> MASSRCPAPRGCRCLPGASLAWLGTVLLLLADWVLLRTALPRIFSLLVPTALPLLRVWAVGLSRWAVLWLGACGVLRA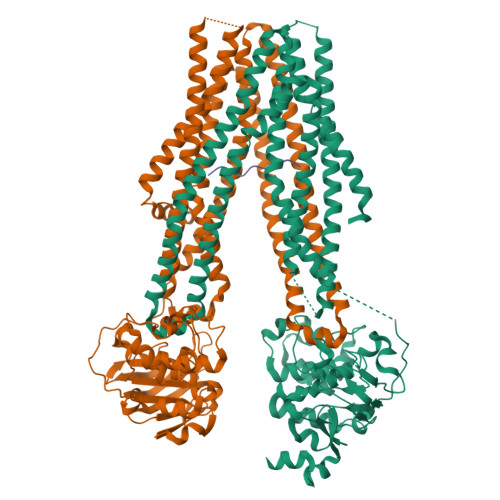TVGSKSENAGAQGWLAALKPLAAALGLALPGLALFRELISWGAPGSADSTRLLHWGSHPTAFVVSYAAALPAAALWHKLGSLWVPGGQGGSGNPVRRLLGCLGSETRRLSLFLVLVVLSSLGEMAIPFFTGRLTDWILQDGSADTFTRNLTLMSILTIASAVLEFVGDGIYNNTMGHVHSHLQGEVFGAVLRQETEFFQQNQTGNIMSRVTEDTSTLSDSLSENLSLFLWYLVRGLCLLGIMLWGSVSLTMVTLITLPLLFLLPKKVGKWYQLLEVQVRESLAKSSQVAIEALSAMPTVRSFANEEGEAQKFREKLQEIKTLNQKEAVAYAVNSWTTSISGMLLKVGILYIGGQLVTSGAVSSGNLVTFVLYQMQFTQAVEVLLSIYPRVQKAVGSSEKIFEYLDRTPRCPPSGLLTPLHLEGLVQFQDVSFAYPNRPDVLVLQGLTFTLRPGEVTALVGPNGSGKSTVAALLQNLYQPTGGQLLLDGKPLPQYEHRYLHRQVAAVGQEPQVFGRSLQENIAYGLTQKPTMEEITAAAVKSGAHSFISGLPQGYDTEVDEAGSQLSGGQRQAVALARALIRKPCVLILDDATSALDANSQLQVEQLLYESPERYSRSVLLITQHLSLVEQADHILFLEGGAIREGGTHQQLMEKKGCYWAMVQAPADAPE;> MRLPDLRPWTSLLLVDAALLWLLQGPLGTLLPQGLPGLWLEGTLRLGGLWGLLKLRGLLGFVGTLLLPLCLATPLTVSLRALVAGASRAPPARVASAPWSWLLVGYGAAGLSWSLWAVLSPPGAQEKEQDQVNNKVLMWRLLKLSRPDLPLLVAAFFFLVLAVLGETLIPHYSGRVIDILGGDFDPHAFASAIFFMCLFSFGSSLSAGCRGGCFTYTMSRINLRIREQLFSSLLRQDLGFFQETKTGELNSRLSSDTTLMSNWLPLNANVLLRSLVKVVGLYGFMLSISPRLTLLSLLHMPFTIAAEKVYNTRHQEVLREIQDAVARAGQVVREAVGGLQTVRSFGAEEHEVCRYKEALEQCRQLYWRRDLERALYLLVRRVLHLGVQMLMLSCGLQQMQDGELTQGSLLSFMIYQESVGSYVQTLVYIYGDMLSNVGAAEKVFSYMDRQPNLPSPGTLAPTTLQGVVKFQDVSFAYPNRPDRPVLKGLTFTLRPGEVTALVGPNGSGKSTVAALLQNLYQPTGGQVLLDEKPISQYEHCYLHSQVVSVGQEPVLFSGSVRNNIAYGLQSCEDDKVMAAAQAAHADDFIQEMEHGIYTDVGEKGSQLAAGQKQRLAIARALVRDPRVLILDEATSALDVQCEQALQDWNSRGDRTVLVIAHRLQTVQRAHQILVLQEGKLQKLAQL;> RRYQKSTEL(4R)-4-[(3S,5R,8R,9S,10S,13R,14S,17R)-10,13-dimethyl-3-(2-methyl-2-oxidanyl-propyl)-2,3,4,5,6,7,8,9,11,12,14,15,16,17-tetradecahydro-1H-cyclopenta[a]phenanthren-17-yl]pentanoic 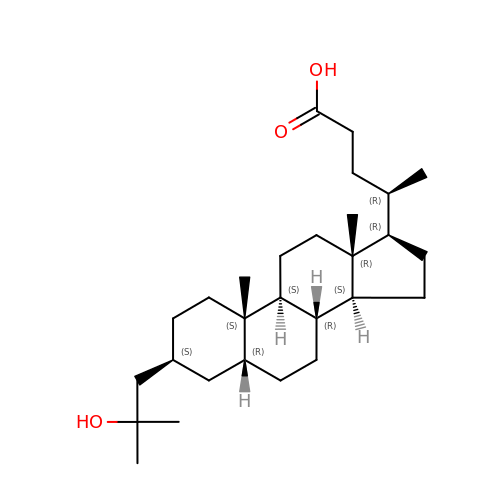acid | C28 H48 O3 | YEJWIEPCSOSHIJ-WDGWKBJASA-N> MSETQSQTMTRPQDLSLSDINSTVEVPEGHSFWKTLLAYSGPGALVAVGYMDPGNWSTSITGGQNFQYL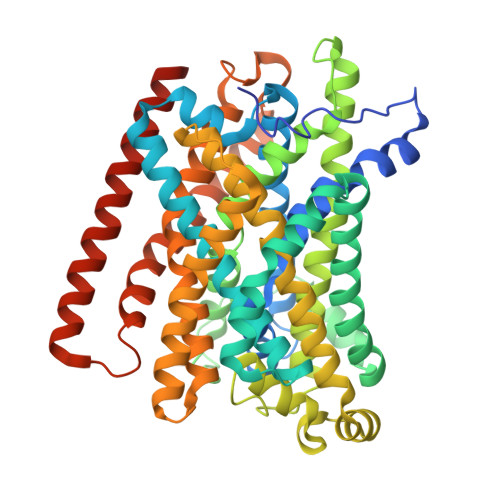LLSIIVISSLLAMLLQNMAAKLGIVCQLDLAQAIRARTSRRLGFIFWILTELAIMATDIAQVIGAAIALYLLFKIPIFLAVVITVLDVFLLLLLNRIGFRKIEALVVCLIFVILFVFLYQIILSQPAWHQVAKGLIPSWASVQTSPKIGGQTPLSASLGIIGATIMPHNLFLHSAISQSRKIDRTDSSKVAEAVRFSNWDSNIQLSLAMVVNALLLIMGVAVFKSGAVQDPSFFGLYQALSNPDMVSNPVLAEAARSGVLSTLFAVALLASGQNSTITGTITGQVIMEGFIHLRLPLWLRRLVTRLIAIIPVVVCVAITSHQGSLDEHQALNNLMNNSQVFLALALPFSIVPLLMLTDSAAQMGNQFKNTRWVKVMGWLTVIILTLLNLISISSQIAGFFGDNPSSQDLLLSQVISIGIILAMIGLLIWTIIDIRRFTHPKQKALEVLFQ>[2x]C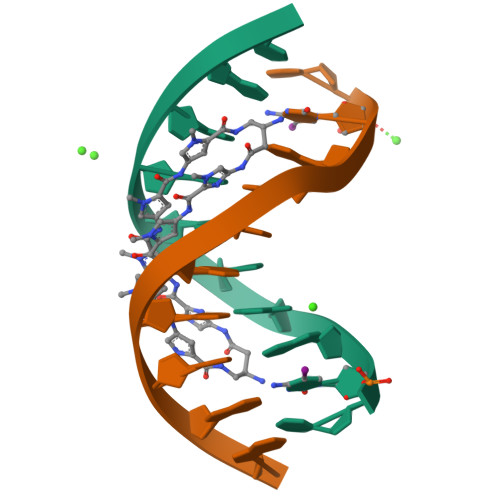CAGTACTGG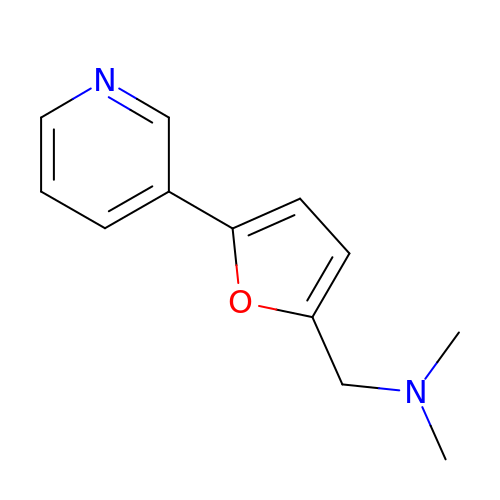N,N-DIMETHYL(5-(PYRIDIN-3-YL)FURAN-2-YL)METHANAMINE | C12 H14 N2 O | PJHSLLRNPASXIS-UHFFFAOYSA-N>[2x]MITPPD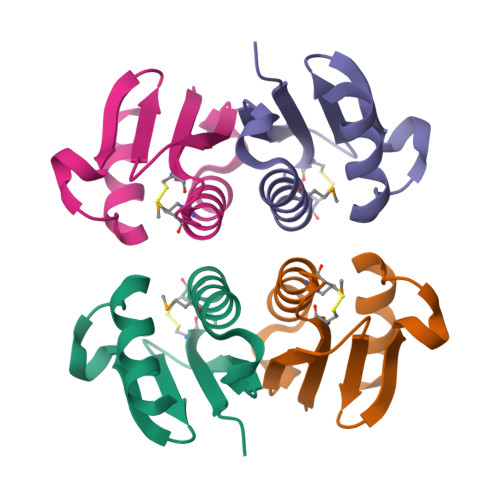HPPRIAIQYCTQCQWLLRAAWMAQELLSTFGADLGEVALVPGTGGVFRIHYNGAPLWDREVDGGFPEAKVLKQRVRDHLDPGRPLGHIDGRPKPLEHHHHHH> MAAHHRQNTAGRRKVQVSYVIRDEVEKYNRNGVNALQLDPALNRLFTAGRDSIIRIWSVNQHKQDPYIASMEHHTDWVNDIVLCCNGKTLISA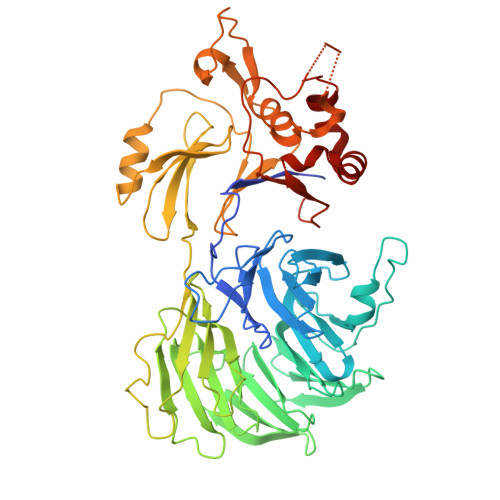SSDTTVKVWNAHKGFCMSTLRTHKDYVKALAYAKDKELVASAGLDRQIFLWDVNTLTALTASNNTVTTSSLSGNKDSIYSLAMNQLGTIIVSGSTEKVLRVWDPRTCAKLMKLKGHTDNVKALLLNRDGTQCLSGSSDGTIRLWSLGQQRCIATYRVHDEGVWALQVNDAFTHVYSGGRDRKIYCTDLRNPDIRVLICEEKAPVLKMELDRSADPPPAIWVATTKSTVNKWTLKGIHNFRASGDYDNDCTNPITPLCTQPDQVIKGGASIIQCHILNDKRHILTKDTNNNVAYWDVLKACKVEDLGKVDFEDEIKKRFKMVYVPNWFSVDLKTGMLTITLDESDCFAAWVSAKDAGFSSPDGSDPKLNLGGLLLQALLEYWPRTHVNPMDEEENEVNHVNGEQENRVQKGNGYFQVPPHTPVIFGEAGGRTLFRLLCRDSGGETESMLLNETVPQWVIDITVDKNMPKFN>[2x]MSGVKVRREDAKKVLELLKSVGILDGKRKAIRDEKYVIFPVTDTNIAKSLGLEVVDVELPMRPERQIYKNLEDLLPREIFKKLGRLDIVGDIAIVSIPDEILSEREVIVSAIRKLYPKVKVIARRGFHSGLYRIRELEVIWGENRLHTIHKENGVLIKVDLSKVFFNPRMKGERYRIAQLVNDGERILVPFAGVIPYPLVIARFKNVEVYAVEINEFAVKLAEENLELNR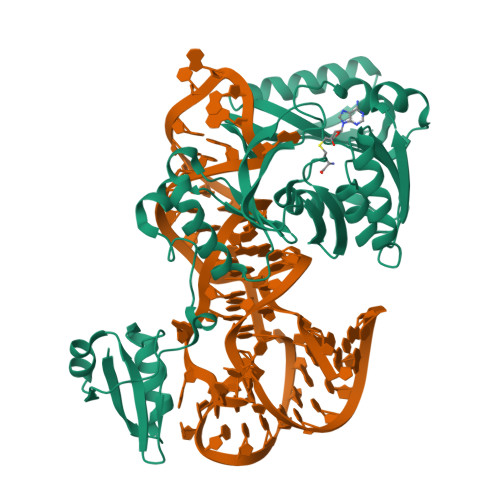DRLKGKIKIIHGDVFEVLPNLPNFDRVVSPTPKGVDALSLTLSKAEKFLHYYDFVHESEIERFRERVLEECRRQGKECRVSVRKVSDYKPHVYKVCADVEILS>[6x]MV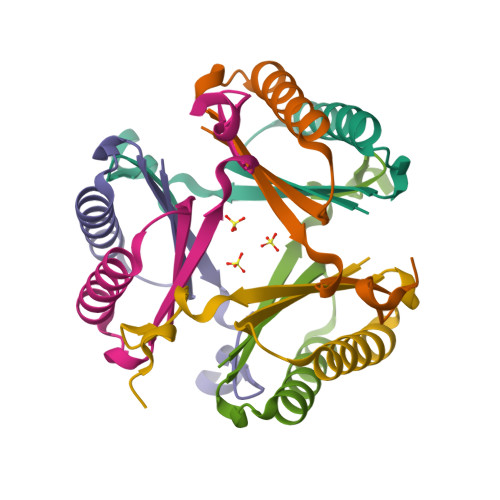VLKVTLLEGRPPEKKRELVRRLTEMASRLLGEPYEEVRVILYEVRRDQWAAGGVLFSDKEGT>MPVVKINAIEVPAGAGPELE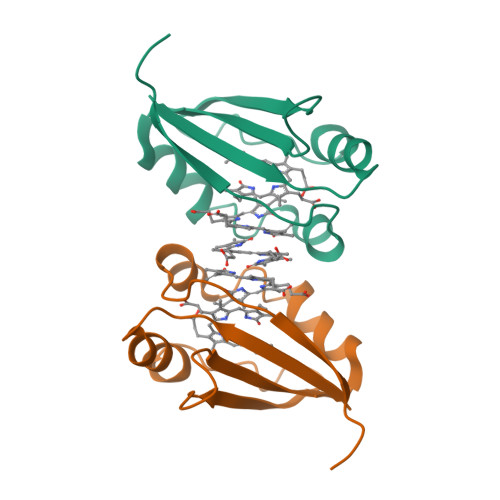KRFAHSAHAVENSPGFLGFQLLRPVKGEERYFVVTHWESDEAFQAWANGPAIAAHAGHRANPVATGASLLEFEVVLDVGGTGKTAGVPRGKLAAALEHHHHHH[2x]Viruses from the family Picornaviridae form non-enveloped icosahedral virions that are about 30 nm in diameter. The capsid proteins VP1, VP2, VP3, and VP4 originating from a single polyprotein form a protomer, the basic building block of the icosahedral capsid. The entire capsid consists of 60 such protomers, arranged in 12 pentamer units. Here we show that the exit of the RNA from the particles of echoviruses 18 and 30 requires capsid opening and results in a loss of up to three adjacent capsid protein pentamers.

The interactions of enteroviruses with receptors or exposure to acidic pH in endosomes induce conformational changes in virions into an activated state characterized by increased particle diameter, reduced contact areas between pentamers of capsid protein protomers, release of VP4 subunits from particles, and externalization of the N termini of VP1 subunits. Receptor binding or exposure to acidic pH induces the transformation of native virions into activated particles with reduced inter-pentamer interfaces. The conversion of echovirus 18 virions to activated particles occurred in <3 min after exposure to acidic pH at 37 °C, however some of the particles also released their RNA and aggregated. The electron density of the genomes is distributed uniformly in echovirus 18 virions at neutral pH, but transforms to a grainy appearance in activated particles at acidic pH. The inter-pentamer contacts of 11,000 Å2 in native echovirus 18 virion are reduced to 5400 Å2 in the activated particles. Correspondingly, the interaction between two pentamers in an activated particle of echovirus 18 is 25% weaker than that in a native virion. The weakening of the inter-pentamer contacts together with the changes in the genome organization, probably enable the opening of the activated particles for genome release. Comparing the cryo-EM images of native virions with activated particles of echovirus 18, as well as other enteroviruses, reveals that their genomic RNAs undergo conformational changes upon exposure to acidic pH. During the shift from neutral to acidic pH, the side chains of histidines of capsid proteins, and probably also parts of the genomic RNA, become protonated, and thus acquire more positive charge. The changes in the charge distribution and putative release of the polyamines from virions may result in the observed changes in the genome structure and increased pressure on the capsid from the inside.

> GDNQDRTVANTQPSGPSNSTEIPALTAVETGHTSQVDPSDTIQTRHVVNFHSRSESTIENFMGRAACVFMDQYKINGEETSTDRFAVWTINIREMAQLRRKCEMFTYMRFDIEMTMVITSCQDQGTILDQDMPVLTHQIMYVPPGGPIPAKVDGYEWQTSTNPSVFWTEGNAPPRISIPFISVGNAYSSFYDGWSHFTQDGTYGYTTLNAMGKLYIRHVNRSSPHQITSTIRVYFKPKHIKAWVPRPPRLCPYINKRDVNFVVTEITDSRTSITDTPHPEHSVLATH;> SPSAEECGYSDRVRSMTLGNSTITTQESANVVVGYGEWPSYLSDREATAEDQPTQPDVATCRFYTLESVQWEKTSPGWWWKFPEALKNMGLFGQNMHYHYLGRAGYTIHVQCNASKFHQGCLLVVCVPEAEMGCADTDTTFPATELTTEDTPHVFTSDSITGKKVQAAVCNAGMGVGVGNLTIFPHQWINLRTNNSATIVIPYINSVPMDNMFRHYNFTLMIIPFAPLNFTDGATAYVPITVTIAPMYAEYNGLRLASTQ;> GVPVLNTPGSNQFLTSDDYQSPSAMPQFDETPEMHIPGEVRNLMEIAEVDSVVPVNNVTGKTKSMDAYQIPVGTGNTDKTKPIFSFQMDPGYSSVLKRTLLGEMLNYYAHWSGSVKLTFLFCGSAMATGKLLISYSPPGASVPTSRKDAMLGTHIVWDIGLQSSCVLCVPWISQSHYRMVQQDPYTSAGYITCWYQTNIVVPPGAPTSCDVLCFASACNDFSVRLLRDTPFMAQPGKLQ> MHKDVKAIYEESKILDEATHLYGVQRSDIHFIADAENYVYELKKDGESFILKITHTIRRSPDYILGEMEWLHHLAKGGLSVAKPIASLNGRDIEQVDDGQGGSFLLRVYEKAPGHKVEEADWNDELFYALGQYTGRMHKLTKSYQLSDPRYKRQEWDEEEQLKLRKYVPADQTLVFEQADRLMEKLAKLPKNQDTYGLVHADLHHGNFHWDQGKITTFDFDDIGYNWFMNDISILLYNVLWYPVIP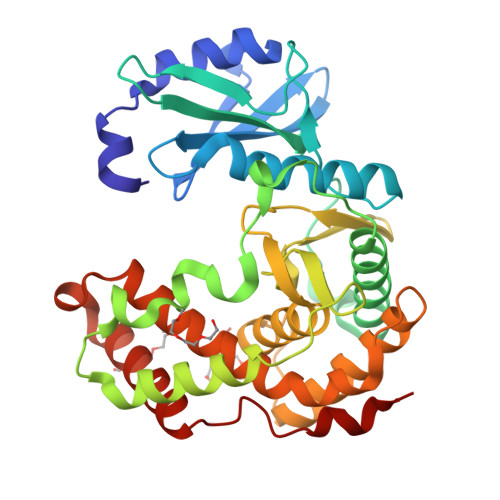YEDKAAFAGNFMKQFLKGYREENELGDEWLAYIPDFLRLRHVLIYGLLHQAFDLATIGDEEKAMLASFRSDIEQAAPITTFDFTKLSQS> GSHMASMTGGQQMGRDPKNVPPLTANQKSLIARLVYYQEGYEQPSEEDLKRVTQTWQSDEDDEDSDMPFRQITEMTILTVQLIVEFAKGLPGFSKISQSDQITLLKACSS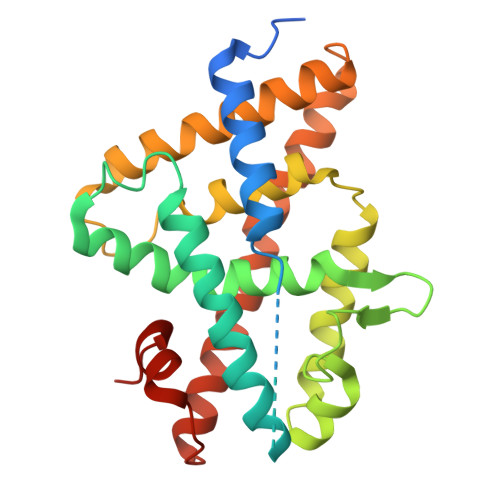EVMMLRVARRYDAATDSVLFANNQAYTRDNYRKAGMAYVIEDLLHFCRCMYSMMMDNVHYALLTAIVIFSDRPGLEQPSLVEEIQRYYLNTLRVYILNQNSASPRSAVIFGKILGILTEIRTLGMQNSNMCISLKLKNRKLPPFLEEIWDVADVA The nap particle is an immunogenic surface adhesion complex from Mycoplasma genitalium. It is essential for motility and responsible for binding sialylated oligosaccharides on the surface of the host cell. Cryo-electron tomography (cryo-ET) of M. genitalium revealed the tetrameric organization of the nap particle complex, consisting of two P140-P110 heterodimers. The P140-P110 heterodimers form the ‘tight interface’, while the ‘loose interface’ is formed between the two heterodimers.

We next used the single particle cryo-EM dataset of the purified nap particles to analyze the C-terminal stalks that connect the crown region with the sialic acid binding pocket to the transmembrane helices and the intracellular domain. For this, we analyzed 290,179 heterodimers which allowed the resolving of both stalk domains which had not been possible before, since previous heterodimer constructs were truncated. After classification, two distinct classes showing both the stalk regions of P110 and P140 were solved at resolutions of 3.3 Å and 3.7 Å, respectively. (a) The canonical purified nap particle heterodimer at 3.3 Å agrees with the crystal and (b) the alternative conformation of the P140 stalk at 3.7 Å displays substantial variations in the P140 stalk region.

> MKTMRKQIYKKAYWLLLPFLPLALANTFLVKEDSKNVTAYTPFATPITDSKSDLVSLAQLDSSYQIADQTIHNTNLFVLFKSRDVKVKYESSGSNNISFDSTSQGEKPSYVVEFTNSTNIGIKWTMVKKYQLDVPNVSSDMNQVLKNLILEQPLTKYTLNSSLAKEKGKTQREVHLGSGQANQWTSQRNQHDLNNNPSPNASTGFKLTTGNAYRKLSESWPIYEPIDGTKQGKGKDSSGWSSTEENEAKNDAPSVSGGGSSSGTFNKYLNTKQALESIGILFDDQTPRNVITQLYYASTSKLAVTNNHIVVMGNSFLPSMWYWVVERSAQENASNKPTWFANTNLDWGEDKQKQFVENQLGYKETTSTNSHNFHSKSFTQPAYLISGIDSVNDQIIFSGFKAGSVGYDSSSSSSSSSSSSTKDQALAWSTTTSLDSKTGYKDLVTNDTGLNGPINGSFSIQDTFSFVVPYSGNHTNNGTTGPIKTAYPVKKDQKSTVKINSLINATPLNSYGDEGIGVFDALGLNYNFKSNQERLPSRTDQIFVYGIVSPNELRSAKSSADSTGSDTKVNWSNTQSRYLPVPYNYSEGIIDADGFKRPENRGASVTTFSGLKSIAPDGFANSIANFSVGLKAGIDPNPVMSGKKANYGAVVLTRGGVVRLNFNPGNDSLLSTTDNNIAPISFSFTPFTAAESAVDLTTFKEVTYNQESGLWSYIFDSSLKPSHDGKQTPVTDNMGFSVITVSRTGIELNQDQATTTLDVAPSALAVQSGIQSTTQTLTGVLPLSEEFSAVIAKDSDQNKIDIYKNNNGLFEIDTQLSNSVATNNGGLAPSYTENRVDAWGKVEFADNSVLQARNLVDKTVDEIINTPEILNSFFRFTPAFEDQKATLVATKQSDTSLSVSPRIQFLDGNFYDLNSTIAGVPLNIGFPSRVFAGFAALPAWVIPVSVGSSVGILFILLVLGLGIGIPMYRVRKLQDASFVNVFKKVDTLTTAVGSVYKKIITQTGVVKKAPSALKAANPSVKKPAAFLKPPVQPPSKPEGEQKAVEVKSEETKSHHHHHH;> MHQPKKRLAKKSWAFLTAALTLGVITGVGGYFLFNQNKQRSSVSNFAYQPKQLSVKHQQAVDETLTPWTWNNNNFSSLKITGENPGSFGLVRSQNDNLNISSVTKNSSDDNLKYLNAVEKYLDGQQNFAIRRYDNNGRALYDINLAKMENPSTVQRGLNGEPIFDPFKGFGLTGNAPTDWNEIKGKVPVEVVQSPHSPNLYFVLLVPKVALEYHNLNNQVVKESLEVKATQSSFNPTQRLQKDSPVKDSSKQGEKLSETTASSMSSGMATSTRAKALKVEVERGSQSDSLLKNDFAKKPLKHKNSSGEVKLEAEKEFTEAWKPLLTTDQIAREKGMGATVVSFYDAPYSENHTAFGLVDHIDPKKMVENYPPSWKTPKWNHHGIWDYNARNLLLQTTGFFNPRRHPEWFDEGQAKADNTSPGFKVGDTDHKKDGFKKNSSSPIALPFEAYFANIGNMVAIGNSVFIFGGNGHATKMFTTNPLSIGVFRIKYTDNFSKSSVTGWPYAVLFGGLINPQTNGLKDLPLGTNRWFEYVPRMAVSGVKWVGNQLVLAGTLTMGDTATVPRLKYDQLEKHLNLVAQGQGLLREDLQIFTPYGWANRPDIPVGAWLQDEMGSKFGPHYFLNNPDIQDNVNNDTVEALISSYKNTDKLKHVYPYRYSGLYAWQLFNWSNKLTNTPLSANFVNENSYAPNSLFAAILNEDLLTGLSDKIFYGKENEFAENEADRFNQLLSLNPNPNTNWARYLNVVQRFTTGPNLDSSTFDQFLDFLPWIGNGKPFSNSPSPSTSASSSTPLPTFSNINVGVKSMITQHLNKENTRWVFIPNFSPDIWTGAGYRVQSANQKNGIPFEQVKPSNNSTPFDPNSDDNKVTPSGGSSKPTTYPALPNSISPTSDWINALTFTNKNNPQRNQLLLRSLLGTIPVLINKSGDSNDQFNKDSEQKWDKTETNEGNLPGFGEVNGLYNAALLHTYGFFGTNTNSTDPKIGFKADSSSSSSSTLVGSGLNWTSQDVGNLVVINDTSFGFQLGGWFITFTDFIRPRTGYLGITLSSLQDQTIIWADQPWTSFKGSYLDSDGTPKSLWDPTALKSLPNSSTTYDTNPTLSPSFQLYQPNKVKAYQTTNTYNKLIEPVDATSAATNMTSLLKLLTTKNIKAKLGKGTASSQGNNNGGGVSQTINTITTTGNISEGLKEETSIQAETLKKFFDSKQNNKSEIGIGDSTFTKMDGKLTGVVSTPLVNLINGQGATSDSDTEKISFKPGNQIDFNRLFTLPVTELFDPNTMFVYDQYVPLLVNLPSGFDQASIRLKVISYSVENQTLGVRLEFKDPQTQQFIPVLNASSTGPQTVFQPFNQWADYVLPLIVTVPIVVIILSVTLGLTIGIPMHRNKKALQAGFDLSNKKVDVLTKAVGSVFKEIINRTGISNAPKKLKQATPTKPTPKTPPKPPVKQ> GSHMHNSNADDAALTTDVVVVGG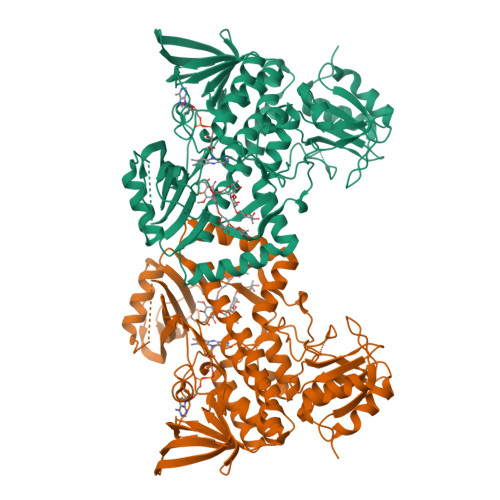GPVGLMLAGELRAGGVGALVLEKLVEPVGHDRAGALHIRTVETLDLRGLLDRFLEGTQVAKGLPFAGIFTQGLDFGLVDTRHPYTALVPQSRTEALLAEHAREAGAEIRRGHEVTGLRQDAEAVEVTVAGPSGPYRVRARYAVGCDGGRSTVRRLAGIGFPGTEATVRALIGYVTTPEREVPRRWERTPDGILVLAFPPEGGLGRVVVIEYTGHSPAADEGPVTLEDLGAAVARVRGTPLTLTEPVSWLSRFGDASRQAKRYRSGRVLLAGDAAHVHFPIGGQGLNTGLQDAVNLGWKLAARVRGWGSEELLDTYHDERHPVAERVLLNTRAQLALMRPDEQHTTPLRGFVEELLGTDEVNRYFTGMITGTDVRYATFAPAAPARPHPWAGRFAGGLVLSGPSGEPVPVAELLRSARPLLLDLAGRADLREATRPWSDRVSVVAGEATVEPPAQALLVRPDGYVAWAGSPAATADELRASLARWFGPPANREPVGHQERAGRRGRPLSALKPE6-[4-[(6-azanylpyridin-3-yl)methylcarbamoylamino]-3-fluoranyl-phenyl]-2-(ethylamino)-~{N}-(2-piperidin-1-ylethyl)pyridine-3-carboxamide 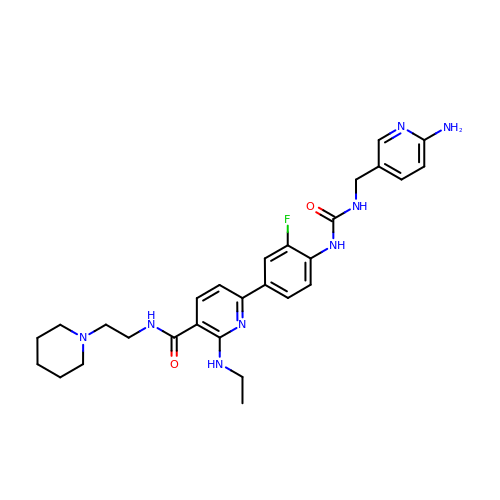| C28 H35 F N8 O2 | JXVZQJNZEWWAKF-UHFFFAOYSA-N CAD is a 1.5 MDa hexameric protein with four enzymatic domains responsible for initiating de novo biosynthesis of pyrimidines nucleotides: glutaminase, carbamoyl phosphate synthetase, aspartate transcarbamoylase (ATC), and dihydroorotase. Moreover, in fungi, GLN, CPS, and ATC are fused into a CAD-like protein with an inactive DHO-like domain, and the DHO activity is encoded as an independent enzyme. The crystal structures of the ATC domains of human CAD and the CAD-like protein from the fungus Chaetomium thermophilum showed a dome-shaped homotrimer with three active sites between the subunits that are very similar to bacterial and plant ATCs. Here, we report the insertion by site-directed mutagenesis of two cysteine (Cys) residues in the ATC domain that favor the formation of disulfide bridges between subunits in the trimer.

So, for this study, we engineered a construct encoding only the ctATC domain (ctATC-WT; aa 1939–2253) fused to a removable N-terminal His6-maltose binding protein (MBP) tag and then introduced the mutations N2045C and R2238C (ctATC2Cys). Using these criteria, we selected residue N2045, in helix α3, and residue R2238, in helix α12. Structural determination by molecular replacement showed one protein subunit per asymmetric unit forming a trimer through the crystallographic threefold axis. The structure of ctATC2Cys is highly similar to that reported for ctATC-WT, as indicated by the low root-mean-square-deviation for the superposition of all Cα atoms in the subunit (rmsd = 0.439 Å) or in the protein trimer (rmsd = 0.704 Å). The high-resolution electron density map was unambiguous and allowed for the building of the entire polypeptide chain, except for residues 2026–2032 that appeared flexibly disordered in the ctATC2Cys apo structure. These missing residues correspond to a loop (the CP-loop) that projects from one subunit into the active site of the adjacent subunit and interacts with the substrate. The only important difference in the structures of ctATC2Cys that are free or bound to CP was the presence of the mutated Cys residues and the extra electron density between their side chains that demonstrates the formation of three disulfide bridges between subunits in the trimer. Thus, we conclude that the Cys and formation of the disulfide bridges do not alter the protein folding or oligomerization and do not interfere with the binding of CP. Instead, the double mutant ctATC2Cys had a Tm = 73.5 °C, 20 °C higher than ctATC-WT, and similar to the Tm of human ATC bound to PALA, which induces a tight and nearly irreversible complex. Extrapolation of the curves to an infinite concentration of the chemical indicated that Cys substitutions increase the Tm by 3–4 °C and that the remainder is due to disulfide bridge formation.

> PLQEMLAAPSSFKKSHVLSVTQFTRADLHLLFQIAQEMRLGVQREGVLDILRGKVLCTLFYEPSTRTSASFDAAMQRLGGRTIPIQTSTSSVQKGETLQDTLRTLACYSDAIVLRHPDEKCVDVAKKYCPVPVINGGNGSKEHPTQAFLDLFTIREELGTMQGLTITFVGDLLYGRPVHSLVYLLRHYQVKVQLVSPKALRLPPAVRQQLVDAGQLLCESEALTPEILGRTDVLYCTRVQKERFPSLAEFEAVKDSYRIDYSTLKYAKPTTVVMHPLPRNEEVAEEVDFDQRAAYFRQMCYGLYCRMALLALVMS> MLYIDEFKEAIDKGYILGDT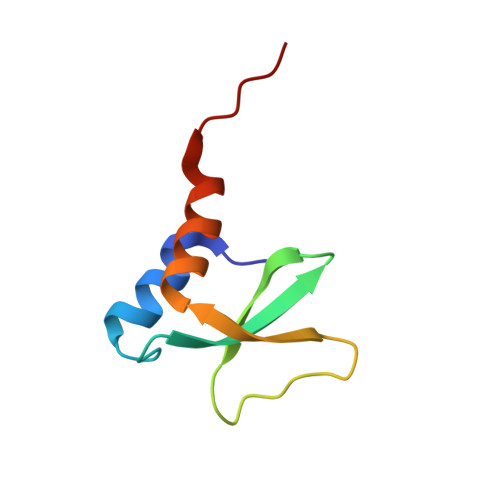VAIVRKNGKIFDYVLPHEKVRDDEVVTVERVEEVMVELDKLEHHHHHH1-(4-TERT-BUTYLCARBAMOYL-PIPERAZINE-1-CARBONYL)-3-(3-GUANIDINO-PROPYL)-4-OXO-AZETIDINE-2-CARBOXYLIC ACID | C18 H33 N7 O5 | 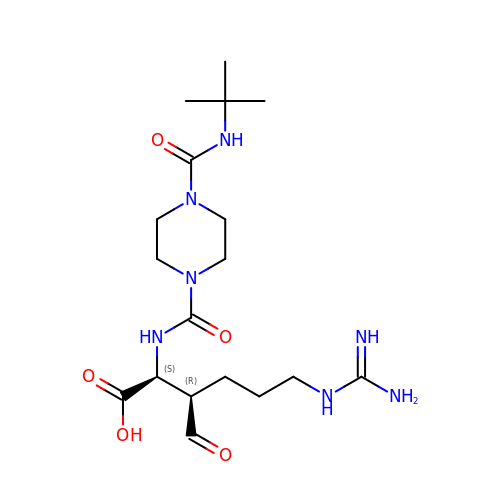BVNQCAHTTOIOEK-STQMWFEESA-N> KMKKILSFDIDNTLNEPKMPIFPEMAELLATLS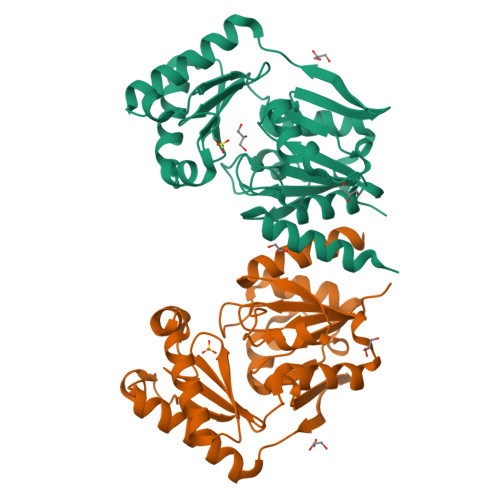QKYIIAPISGQKYDQFLIQIINNLPESANLDNFHLFVAQGTQYYAHKAGEWKQVFNYALTDEQANAIMGALEKAAKELGHWDESVLLPGDEINENRESMIAYSAIGQKAGVEAKQAWDPDMTKRNEIAKLASQYAPEFEFEVAGTTTINGFVPGQNKEFGMNHLMEELNVTKEEILYFGDMTQPGGNDYPVVQMGIETITVRDWKETAAILKAIIAMEEA;> AMKKILSFDIDNTLNEPKMPIFPEMAELLATLSQKYIIAPISGQKYDQFLIQIINNLPESANLDNFHLFVAQGTQYYAHKAGEWKQVFNYALTDEQANAIMGALEKAAKELGHWDESVLLPGDEINENRESMIAYSAIGQKAGVEAKQAWDPDMTKRNEIAKLASQYAPEFEFEVAGTTTINGFVPGQNKEFGMNHLMEELNVTKEEILYFGDMTQPGGNDYPVVQMGIETITVRDWKETAAILKAIIAMEEA> MGSSHHHHHHSSGTGSGLVPRGSHMSLSKKRKLESGDSGGAGAGGEGAEEENGGEQEAAPPRPRRTKSERDQLYYECYSDVSVHEEMIADQVRTEAYRLGILKNWAALRGKTVLDVGAGTGILSIFCAQAGARRVYAVEASAIWQQAREVVRLNGLEDRVHVLPGPVETVELPERVDAIVSEWMGYGLLHESMLSSVLHARTKWLKEGGLLLPASAELFVAPISDQMLEWRLGFWSQVKQHYGVDMSCMESFATRCLMGHSEIVVQDLSGEDVLARPQRFAQLELARAGLEQELEAGVGGRFRCSCYGSAPLHGFAVWFQVTFPGGDSEKPLVLSTSPLHPATHWKQALLY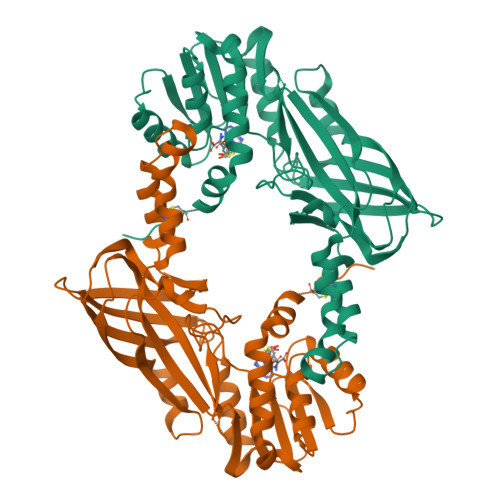LNEPVPVEQDTDISGEITLLPSPDNPRRLRILLRYKVGDHEEKTKDFAMED> MVLIDMSVDLSTQVVDHYENPRNVGSLDKTSKNVGTGLVGAPACGDVMKLQIQVDEKGKIVDARFKTFGCGSAIASSSLATE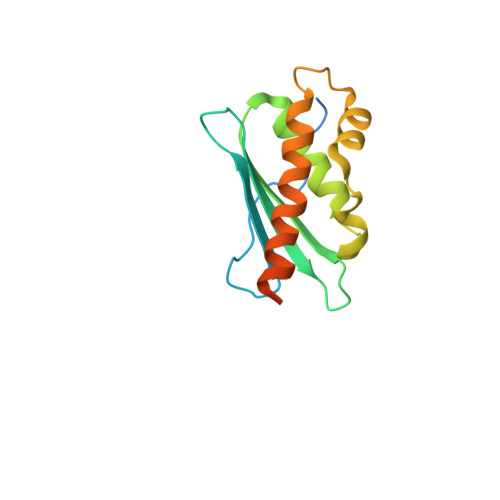WVKGKTVEEALTIKNTDIAKELCLPPVKLHCSILAEDAIKAALADYKLKQEPKKGEAEKKLEHHHHHH> MQVLNTKSETKQENEGSQPPYIQERLKSLNDI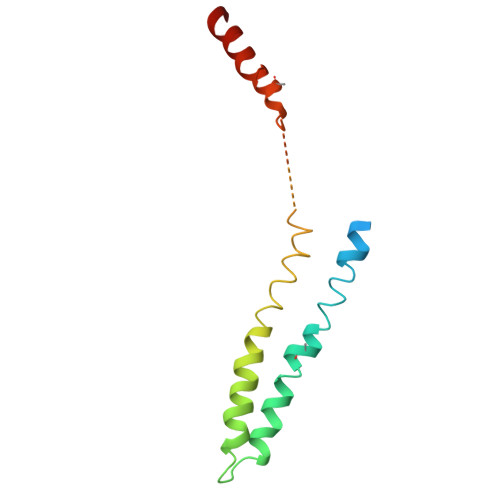ETQLCSMLQEASQVTFIFGELKRGNESVKPQFENHVKQFYERLDKSTTQLRKEIQLLDENVGTRLLPINVNKKALGQDTEKMEEQLDLLSAILDPSKSK>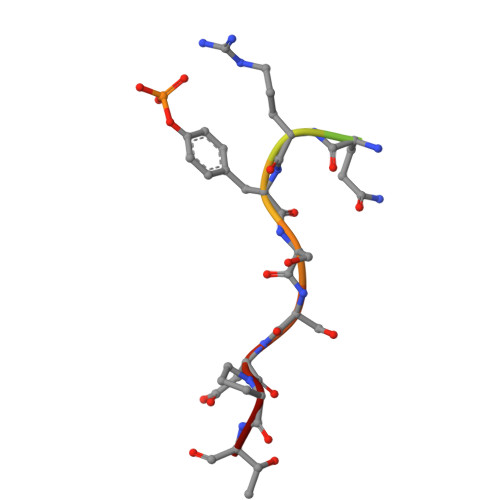 EDSFLQRYSSDPT RTX adhesins are long, multi-domain proteins present on the outer membrane of many Gram-negative bacteria. To expand the reach of the ligand-binding domains, RTX adhesins maintain a central extender region of multiple tandem repeats, which makes up most of the proteins’ large molecular weight. In this study, we analyzed extender regions from two additional RTX adhesins, including the long adhesion proteins from Marinobacter hydrocarbonoclasticus (MhLap) – an oil-eating marine bacterium – and Aeromonas hydrophila (AhLap) – an opportunistic pathogen of fish and mammals. However, all the tetra-tandemers have at least one calcium ion coordinated in the linker region between beta-sandwich domains whose role appears to be the rigidification of the extender region to help the adhesin extend its reach.

Calcium SAD phasing (Guo et al., 2019a, Guo et al., 2019b) was used to solve the tetra-tandemer structures to 2.0 Å (MhLap) and 1.75 Å resolution (AhLap). The repeats are rotated relative to each other around the long central axis, producing a handedness to the tetra-tandemers reminiscent of helices. Both the MhLap and AhLap structures show right-handed rotations, with pitches of approximately i + 3 and i + 2, respectively. The 45 Å-long MhLap repeats are similar yet simpler, keeping the two antiparallel beta sheets but lacking the ancillary structural elements present in MpIBP (i.e. the short sheet, and the helices). Regarding Ca2+ coordination, the MhLap tetra-tandemer is once again the simplest of the three. While the MpIBP tetra-tandemer was found to have many Ca2+ coordinated throughout its structure, MhLap consigns its calcium ions to the linker regions, with only one ion per domain interface. Each calcium in the MhLap tetra-tandemer structure is bound in a similar manner, forming an octahedral coordination sphere comprised of five protein contacts and one water molecule. The protein contacts are made by the sidechains of one asparagine and three aspartate residues, as well as a single backbone carbonyl. Taken together, these spectra demonstrate that the MhLap tetra-tandemer develops into a beta-strand-dominated structure upon Ca2+ addition, although some structure is present in the absence of calcium. To analyze the potential rigidifying properties of these interstitial calcium ions, molecular dynamics simulations on a di-tandemer of the MhLap were undertaken with and without the Ca2+ present. The di-tandemer maintained a rod-like structure, with the Bend angle between the two domains never deviating over 30° relative to the start frame; the two domains saw slightly more twisting over the simulation, maintaining a ~ 60° wedge.

> MASSHHHHHHSSGLVPRGSHMSFDATAGALTVSLDTVDNTAQTANLSGTTTDVAPNEQVAITITDSAGNIVNAIATVGADGSYSLTGVDISSLVDGSLTVEASAQDRNGNALTDSANGALDATAGDLTVSVGTIDNTAQTVNLSGTTTDVAPNGQVAITMTDSAGNIVNATATVGADGSYSLTGVDISSLVDGDLTVEASAQDRNGNAVSDSANGTFDATAGDLTVSVDTVDSTAQTANLSGTTTDVALNSQVDLTVTDSAGNVVTATTTVGADGSYSLTGVDISSLVDGNLTVEATAQDRNGNAVSDSAAGSLDATTGALTVSLDTVDNAAQTVDLSGTTADVAPNSQVNVTITDSTGNVVNAITTVGADGSYSLTGVDISSLVDGDLTVEASAQGRNGNALTDSANGALDAT> AGSVDTVSLYSGRGANMPFTIMEAESTSNATNGTKLTPNFKPGDYAGEASGRSSVYLDATGEYVEFTLTSPANAFVLRNAVAENTTGTVSIYADGVSKGKFNVSSKFSYLYATPSTLGRLGYDNAPGAGLTAYWLYEDAQLMLDQVYPAGTKIKIQKDAGDVSWIYVDLLETENVAPPQANPDPTKYVAVSASKSIDQALTEF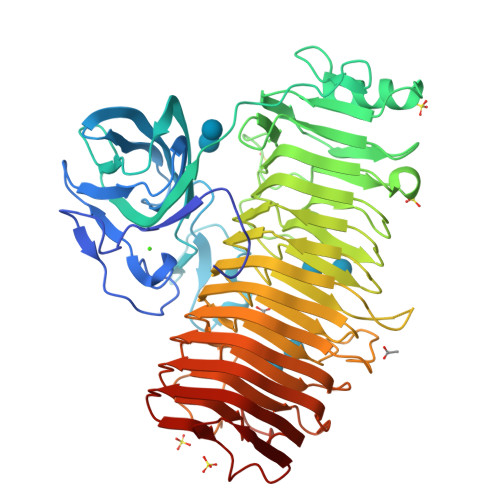RQDNTKKGIYIPAGEWTINSKIFLYGRATEIVGAGPWYTKLVAPQSQSNTDVGFNISAAANGSTIRDLSAWGNYINRVDGPGKFIDGNGMQNVTVQNIWVEHFVCLYWGVNSSYNTFKNNRIKNTFADGINMTNGSSYNVIDNNYARGTGADSFALFSATDSGGSYNVGNKYTNLTATNVRRAAAFAVYGGSDNLFQNLYGADTLTYPGITISSYSFGYNTLGFGDQDTVIDGATLDRTGGDFWTSVGADDKINEYQNFGAIWIYGGDRAIKNILIKNVDINNPVYFGLMFQSMSPNNMVMQNIRVENVNINNPSRYGIKLVVRAEQGQGPAYGGASFTNVKVNNPGISAIYGEAQSPNFTVTRVSGNNW(2,2-dimethyl-2,3-dihydro-1-benzofuran-7-yl)methanol | C11 H14 O2 | 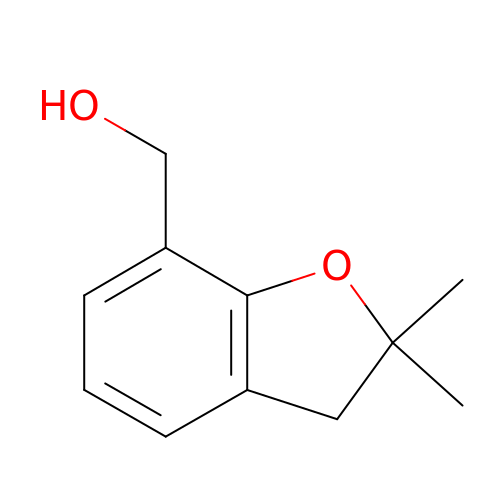LKFXMRFTJVYQMT-UHFFFAOYSA-N> SSSPKITARWNPSEACRPLVDDAPIFYPTNEDFDDPLGYIEKLRSKAESYGICRIVPPVAWRPPCPLKEKKIWENSKFPTRIQFIDLLQNREPIKKSTKTKKRKRRRISKIGYTRRKRDSGCDTASSGSSDSEGKFGFQTGPDFTLAAFQKYDEYFKECYFQSEDHPGSKASENKKFKPKVKDLEGEYWRIVEQATDEVEVYYGADLETKKFG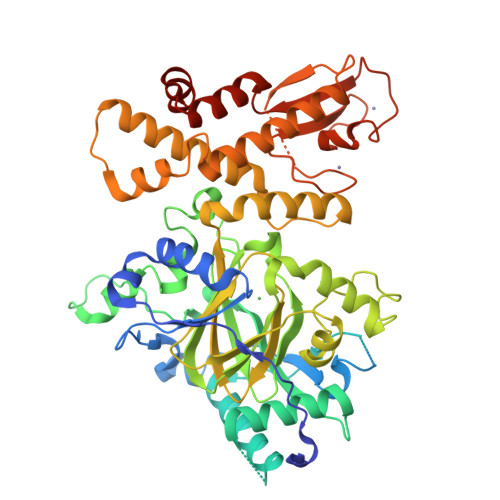SGFPKYKPGYPISEADQYSQCGWNLNNLSRLPGSVLAFESCDISGVIVPWLYVGMCFSTFCWHVEDHHLYSMNYLHTGDPKVWYGIPGNHAESFENVMKKRLPDLFEEQPDLLHQLVTQLSPRILKEEGVPVYRAVQRSGEFILTFPKAYHSGFNCGFNCAEAVNVAPVDWLVHGQNAVEGYSKQRRKSSLSHDKLLLGAAMEATYCLWELSLSKKKTPVIARWKRVCSEDGLLTKAVKKRVQMEEERLNHLQDGFSLRKMEGDFDNKRERECFLCFYDLHMSASSCKCSPNRFACLIHAKDLCSCESKDRYILIRHTLDELWALVRALEGDLDAIDLWASKCRDQYPSQH Reversal of PARylation is predominantly carried out by poly(ADP-ribose) glycohydrolase (PARG) in nucleus and cytosol, whereas ADP-ribosylhydrolase 3 (ARH3) may play a role in mitochondrial PAR degradation. PARG comprises an N-terminal regulatory/targeting domain and a C-terminal catalytic domain. The mouse PARG catalytic domain has a bean-shaped structure, with the active site in a deep cleft in the middle on the abdominal side.

To understand what caused the activity difference between the mPARG E748N/Q and E749N/Q mutants, we solved the crystal structures of these mPARG mutants. Interestingly, while E748N and E749N mutants were completely dead, both E748Q and E749Q mutants still retained residual PARG activities. PARG E748Q and E749Q mutants have very similar conformation in the active site, consistent with the fact that glutamine has the similar size of side chain with glutamate. To study the enzymatic mechanism of mPARG, we tried to soak the catalytic residue Glu748, Glu749 mutants E748N, E748Q, E749N and E749Q with the iso-ADPr, which may be the smallest PARG substrate containing the α(1→2) ribose-ribose glycosidic bond to be cleaved by PARG. In all above four PARG mutant crystal structures, we were not able to observe the electron density for iso-ADPr at the “active” site of mPARG. For the E748Q and E749Q mutants, this may result from the partial catalytic activities of these mutations and/or the low affinity between PARG and iso-ADPr. Surprisingly, we repeatedly observed electron densities, in an unexpected position, which fit well with the chemical structure of iso-ADPr and refined well when iso-ADPr was built into the densities. In these structures, iso-ADPr sits at the secondary binding site which is far away from the cleft. This secondary binding site is at the mouse PARG exon 5 coded region, and is not formed due to crystal packing as it is far away from any PARG region involved in crystal packing. There are four residues (R478, D480, F491 and T493) directly interacting with iso-ADPr.

>[2x]GNLPPEKKWLGTPIEEMRKMPRCGIHLPSLRPSASHTVTVRVDLLRAGEVPKPFPTHYKDLWDNKHVKMPCSEQNLYPVEDENGERTAGSRWELIQTALLNKFTRPQNLKDAILKYNVAYSKKWDFTALVDFWDKVLEEAEAQHLYQSILPDMVKIALCLPNICTQPIPLLKQKMNHSVTMSQEQIASLLANAFFCTFPRRNAKMKSEYSSYPDINFNRLFEGRSSRKPEKLKTLFCYFRRVTEKKPTGLVTFTRQSLEDFPEWERCEKPLTRLHVTYEGTIEGNGRGMLQVDFANRFVGGGVTGAGLVQEQIRFLINPELIVSRLFTEVLDHNECLIITGTEQYSEYTGYAETYRWARSHEDGSEKDDWQRRCTEIVAIDALHFRRYLDQFVPEKVRRELNKAYCGFLRPGVPSENLSAVATGNWGCGAFGGDARLKALIQILAAAAAERDVVYFTFGDSELMRDIYSMHTFLTERKLDVGKVYKLLLRYYNEECRNCSTPGPDIKLYPFIYHAVESSAET> PSASEEQVAQDTEEVFRSYVFYRHQQEQEAE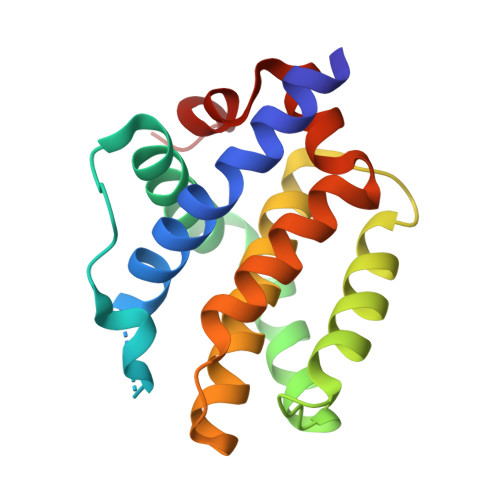GVAAPADPEMVTLPAQPSSTMGQVGRQLAIIGDDINRRYDSEFQTMLQHLQPTAENAYEYFTKIATSLFESGINWRRVVALLGFGYRLALHVYQHGLTGFLGQVTRFVVDFMLHHCIARWIAQRGGWVAALNLGNG> DDSQIKKADATSVAVDASISAFPKKMGPPQWPFSTQYELIGKGVRCVSSITFKAYGLGIYVAAEDKHLVSEVLDSKFLSQAFIDTAAPPSPENSHQDNLRAALNDPAKAPILINNLLDSGIRLMSKNTPIKAGSFKLLMDGTKKSVLKNPDSQSQDKDRLEAGFQELHDCFRSVKGLVARDDDFFIELNKDCSMNLSYYARKKDEFVILGTVKEPLIGKLLFAHYLAAVDPPSPEARKEVIDALVSLS

Saccharomyces cerevisiae possesses two predicted CHI-like proteins, Aim18p (encoded by YHR198C) and Aim46p (YHR199C), but it lacks other enzymes of the flavonoid pathway, suggesting that Aim18p and Aim46p employ the CHI fold for distinct purposes. Here, we demonstrate using proteinase K protection assays, sodium carbonate extractions, and crystallography that Aim18p and Aim46p reside on the mitochondrial inner membrane and adopt CHI folds, but they lack select active site residues and possess an extra fungal-specific loop. Consistent with these differences, Aim18p and Aim46p lack CHI activity and also the fatty acid–binding capabilities of other CHI-like proteins, but instead bind heme. We further show that diverse fungal homologs also bind heme and that Aim18p and Aim46p possess structural homology to a bacterial hemoprotein.

Full-length constructs of Aim18p and Aim46p possessing N-terminal 8X-His tags were insoluble, but truncating the N-terminal mitochondrial targeting sequence and transmembrane domain for Aim18p and Aim46p (Aim18p-Nd70 and Aim46p-Nd62, respectively) dramatically increased solubility. Additionally, the structure of Aim46p-Nd62-WT contained a small molecule resembling α-ketoglutarate in the active site (Document S2), but we were unable to confirm its identity via mass spectrometry. Despite multiple attempts, we were unable to generate heme-bound crystal structures for either Aim18p or Aim46p. Alignments of the Aim18-Nd70-R123A and Aim46-Nd62-WT structures with the bacterial protein revealed that, while the α-helices differed substantially, the core CHI antiparallel β-sheet was structurally homologous to the core antiparallel β-sheet of cytochrome c'β-Met. Of note is a region of the Aim18p-Nd70 and Aim46-Nd62 structures that lies in between plant CHI α1 and α2. This region contains an extra loop that is absent in plant CHI domain–containing proteins but is conserved across multiple ascomycete Aim18p and Aim46p homologs. Nearly all of the CHI catalytic residues are substituted nonconservatively in Aim18p and Aim46p except for the catalytic arginine, which is invariably conserved in fungal homologs of Aim18p and Aim46p. A single nonconservative mutation in these residues is sufficient to nearly abolish catalytic activity, so the presence of several substitutions suggests that Aim18p and Aim46p likely lack canonical CHI enzymatic activity. Upon treatment with sodium carbonate, Aim18p was liberated into the soluble fraction, while a significant proportion of Aim46p remained in the insoluble fraction, suggesting that Aim46p′s transmembrane domain might be more strongly associated with the IMM.>MHHHHHHGSTLYKKAGFEGDRTMIEFDNLTYLHGKPQGTGLLKANPEDFVVVEDLGFEPDGEGEHILVRILKNGCNTRFVADALAKFLKIHAREVSFAGQKDKHAVTEQWLCARVPGKEMPDLSAFQLEGCQVLEYARHKRKLRLGALKGNAFTLVLREVSNRDDVEQRLIDICVKGVPNYFGAQRFGIGGSNLQGAQRWAQTNTPVRDRNKRSFWLSAARSALFNQIVAERLKKADVNQVVDGDALQLAGRGSWFVATTEELAELQRRVNDKEL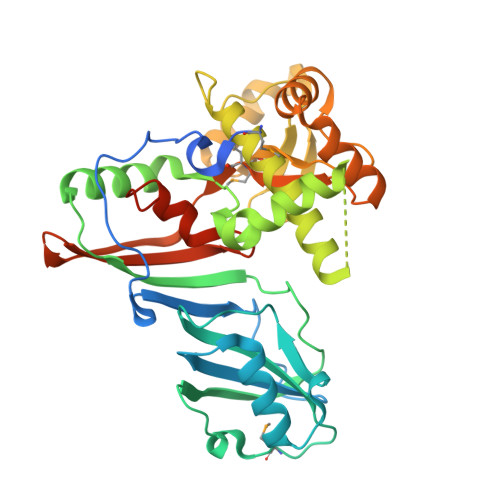MITAALPGSGEWGTQREALAFEQAAVAAETELQALLVREKVEAARRAMLLYPQQLSWNWWDDVTVEIRFWLPAGSFATSVVRELINTTGDYAHIAESTHHHHHH[2x]> MKTAWVFPGQGSQAVGMGVDLLSTAIAKEKYQQAEEILGWSVVEKCQGDEASLALTQNTQPCLYVIEAILADLLRDKGFQPDYVAGHSLGEYSALYAAGVFDFATGLQLVKQRSEVMASASGGMMAALMKFDQTQLQQALTDNTEVVLANDNSPEQVVISGTVAGVEAILANVKARRAVPLKVSG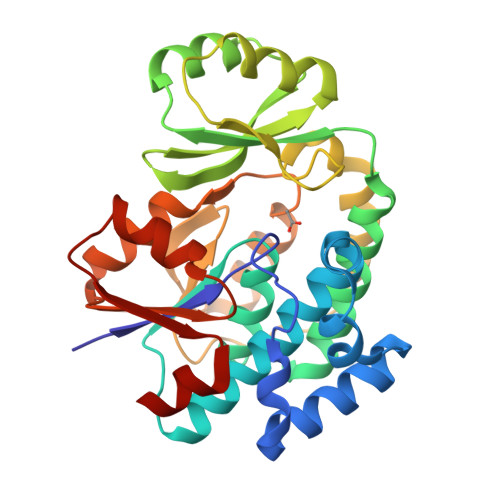AFHSSFMAQPSQSFAQTLTACHFNDATVPVLSNVDPSPTQNGDRLKEKLIQQMTGSVRWRETMVNLGEIGATDYWEVGPGKVLTGLCKRTCPDLNLKNIGQLDDLNSL>MHHHHHHGMASMTARPLSELVERGWAAALEPVADQVAHMGQFLRAEIAAGRRYLPAGSNVLRAFTFPFDNVRVLIVGQDPYPTPGHAVGLSFSVAPDVRPWPRSLANIFDEYTADLGYPLPSNGDLTPWAQRGVLLLNRVLTVRPSNPASHRGK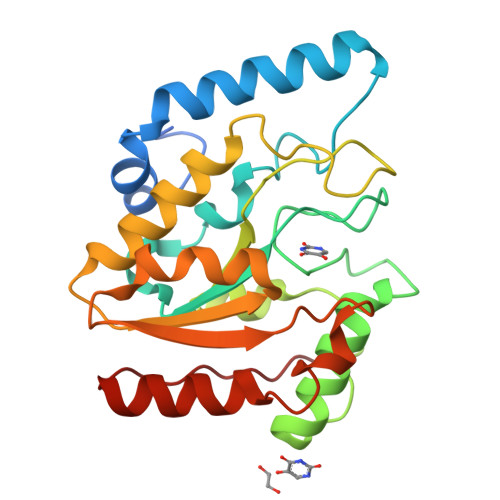GWEAVTECAIRALAARAAPLVAILWGRDASTLKPMLAAGNCVAIESPHPSPLSASRGFFGSRPFSRANELLVGMGAEPIDWRLP[2x]> MTNYTVDTLNLGEFITESGEVIDNLRLRYEHVGYHGQPLVVVCHALTGNHLTYGTDDYPGWWREII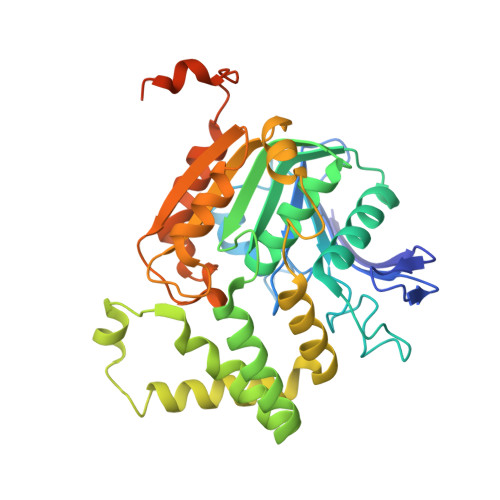DGGYIPIHDYQFLTFDVIGSPFGSSSPLNDPHFPKKLTLRDIVRANERGIQALGYDKINILIGGSLGGMQAMELLYNQQFEVDKAIILAATSRTSSYSRAFNEIARQAIHLGGKEGLSIARQLGFLTYRSSKSYDERFTPDEVVAYQQHQGNKFKEHFDLNCYLTLLDVLDSHNIDRGRTDVTHVFKNLETKVLTMGFIDDLLYPDDQVRALGERFKYHRHFFVPDNVGHDGFLLNFSTWAPNLYHFLNLKHFKRKDPAFLYKVVINSKLEGKPIPNPLLGLDSTRTGHHHHHH One such quadruplex-forming sequence is found in the promoter region of the human c-MYC oncogene. c-MYC is estimated to be dysregulated or overexpressed in approximately 70% of all human cancers and is responsible for mediating multiple pathways important in tumor cell survival. Stabilization of the major quadruplex formed in the c-MYC promoter by various small molecules has been shown to inhibit transcription of c-MYC thereby reducing expression of the oncogene. The human c-MYC promoter quadruplex is formed under negative supercoiling conditions in the nuclease hypersensitivity element III1 region (NHE III1). NHE III1 contains 20 guanines grouped into five segments of 3 to 4 guanine nucleotides separated by one or two adenine or thymine nucleotides. This guanine-rich character allows formation of four possible quadruplex topologies, with the major form being a parallel intramolecular quadruplex comprised of the four guanine segments at the 3’-end of the sequence.

In a previous NMR study, it was found that the major biologically relevant conformation adopted by the c-MYC promoter quadruplex could be selected from other conformers by mutating residues G4, G14 and G23 to thymines and truncating the sequence to 22 nucleotides in length (Pu22). The 22 residue c-MYC promoter sequence Pu22 crystallized in the P21212 space group in a stacked dimer formation with two parallel, single-stranded quadruplex structures per asymmetric unit. Each individual quadruplex contains three loops and a 5’-head and 3’-tail region. The 5’-head region consists of residues T1-G2-A3 and is observed stretched away from the central G-quartets with the residues roughly orthogonal relative to the core guanines. The 3’-tail regions of the two quadruplexes in the asymmetric unit are comprised of residues T20-A21-A22 and are positioned below and approximately planar to the central G-quartets. The quadruplex structure also contains three double-chain reversal propeller-type loops, with two consisting of single thymine residues (T7, T16) that flank a third, two-residue loop (T11-A12). Each individual quadruplex contains two potassium ions at the centers of two stacked G-quartets and an additional potassium ion similarly positioned at the interface that forms the dimer in the asymmetric unit, for a total of five potassium ions in the central cavity. An additional potassium ion is positioned between two adjacent symmetry-related strand B quadruplexes, interacting with O4 oxygen of T7 of one and backbone phosphate of G9 of the other. The two quadruplex strands, A and B, π–π stack together at the G-quartets near their 5’-ends with the G-quartets containing residues G4, G8, G13, and G17 of each quadruplex interacting to create the extended dimer structure.

>[2x]TGAGGGTGGGTAGGGTGGGTAA> GDSIEDKNARVIELIAAYRNRGHLMADIDPLRLDNTRFRSHPDLDVNSHGLTLWDLDREFKVDGFAGVQRKKLRDILSVLRDAYCRHVGVEYTHILEPEQQRWIQERVETKHDKPTVAEQKYILSKLNAAEAFETFLQTKYVGQKRFSLEGAETVIPMMDAVIDQCAEH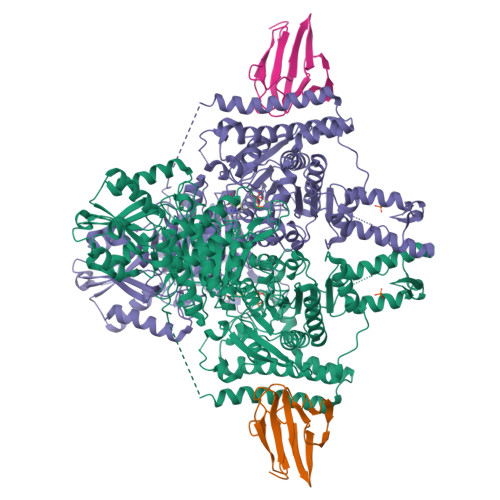GLDEVVIAMPHRGRLNVLANIVGKPYSQIFSEFEGNLNPSQAHGSGDVKYHLGATGTYIQMFGDNDIEVSLTANPSHLEAVDPVLEGLVRAKQDLLDTGEEGSDNRFSVVPLMLHGDAAFAGQGVVAETLNLALLRGYRTGGTIHIVVNNQIGFTTAPTDSRSSEYCTDVAKMIGAPIFHVNGDDPEACAWVARLAVDFRQAFKKDVVIDMLCYRRRGHNEGDDPSMTQPYMYDVIDTKRGSRKAYTEALIGRGDISMKEAEDALRDYQGQLEAVFNEVRELEKHEIEPSESVEADQQIPSKLATAVDKAMLQRIGDAHLALPEGFTVHPRVRPVLEKRREMAYEGRIDWAFAELLALGSLIAEGKLVRLSGQDTQRGTFTQRHAVIVDRKTGEEFTPLQLLATNPDGTPTGGKFLVYNSALSEFAAVGFEYGYSVGNPDAMVLWEAQFGDFVNGAQSIIDEFISSGEAKWGQLSDVVLLLPHGHEGQGPDHTSGRIERFLQLWAEGSMTIAMPSTPANYFHLLRRHGKDGIQRPLIVFTPKSMLRNKAAVSDIRDFTESKFRSVLEEPMYTDGEGDRNKVTRLLLTSGKIYYELAARKAKENREDVAIVRIEQLAPLPRRRLAETLDRYPNVKEKFWVQEEPANQGAWPSFGLTLPEILPDHFTGLKRISRRAMSAPSSGSSKVHAVEQQEILDTAFG;> GSGVEGLPSGSALLVVKRGPNAGSRFLLDQPTTSAGRHPDSDIFLDDVTVSRRHAEFRLEGGEFQVVDVGSLNGTYVNREPVDSAVLANGDEVQIGKFRLVFLTGPKSDDSGSNA6-benzyl-3-[(2R)-2-(3-fluoropyridin-2-yl)-6-methyl-3,4-dihydro-2H-1-benzopyran-7-yl]-4,6-dihydropyrido[4,3-d]pyrimidine-2,7(3H,8H)-dione 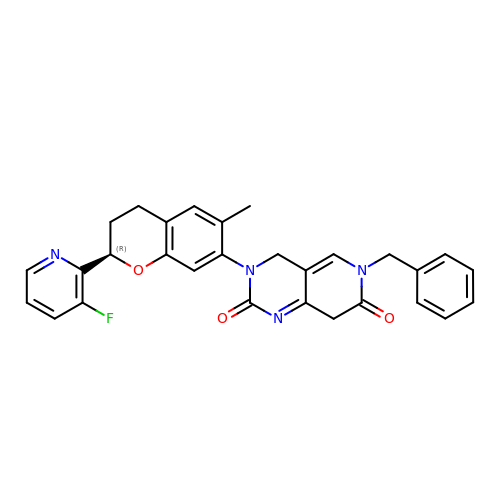| C29 H25 F N4 O3 | IHLUBSALJUDYDX-RUZDIDTESA-N> GSHMTDLPRLPFDNPDIMGIAPQ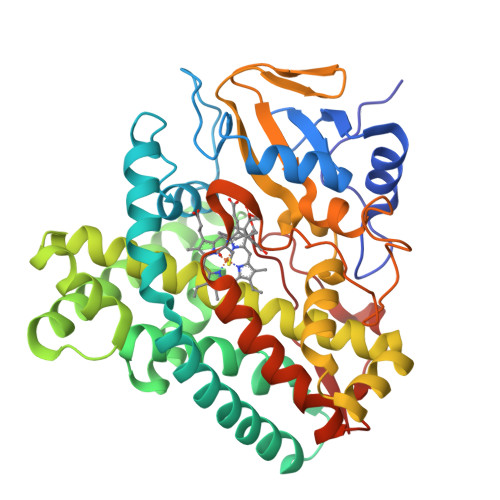MLALQKEGPIARVGTAGEDAWLVTRYDEVRTLLADRRLRLSNPNPQPSAKSAARAFMVALAAGDDHETEPARHAQMRSLLIPRFSTRRLRLMKTRIEHHVDELLDQLAASAPPVDLHRVLSFRLPTMVVCDLLGVPLADRERFGQWARGTFDQSDNEHSANTFQQVVDYMLELVARKRVEPGDDILSELIAEKDGALSDADIAHLGNAVLLFGYETTIVRIDLGTLLLLRNPVQRAQLAEDPGLAPAAVEEILRLGVGGKGSNALIPRYAHGDITVGETVIRTGDAVMLAIGAANYDDRAFPDGGLFDLTRVRPRSHLAFGHGARHCIGRTLARIELTAVFERLFRRLPDLRLAVPEESLRWQEHRITGGFDEIPVTF>[2x]GATCLSQYCADKARDGVCDEACNSHACQWDGGDCSLTMENPWANCSSPLPCWDYINNQCDELCNTVECLFDNFECQGNSKTCKYDKYCAD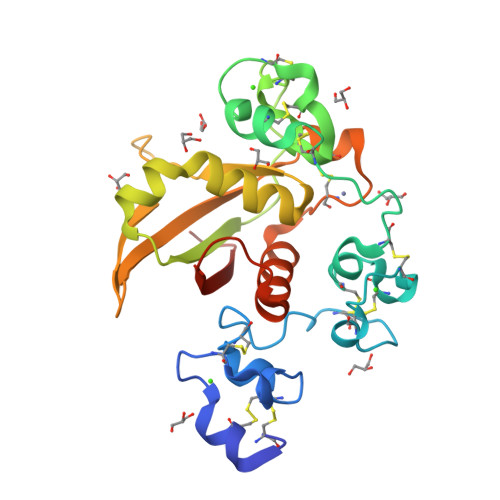HFKDNHCNQGCNSEECGWDGLDCAADQPENLAEGTLVIVVLMPPEQLLQDARSFLRALGTLLHTNLRIKRDSQGELMVYPYYGEVAGSKVFLEIDNRQCVQDSDHCFKNTDAAAALLASHAIQGTLSYPLVSVVSESLTPERTQ(1S,3S,4S)-3-amino-4-(fluoromethyl)cyclopentane-1-carboxylic 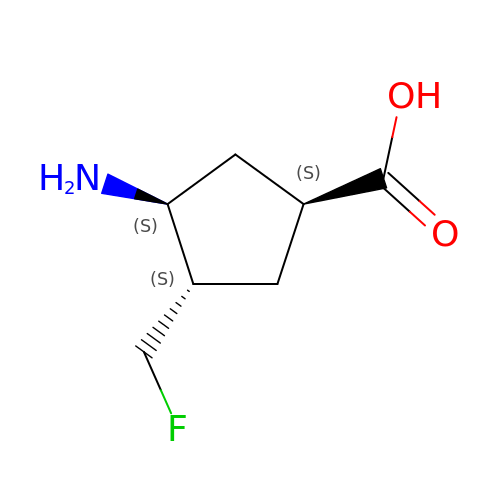acid | C7 H12 F N O2 | ZROKQRHEXPQFAI-JKUQZMGJSA-N> SNAMDLQLSKRLQKVANYVPKGARLLDVGSDHAYLPIFLLQMGYCDFAIAGEVVNGPYQSALKNVSEHGLTSKIDVRLANGLSAFEEADNIDTITICGMGGRLIADILNNDIDK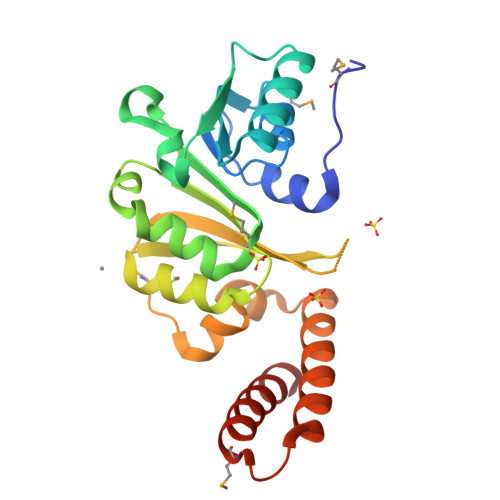LQHVKTLVLQPNNREDDLRKWLAANDFEIVAEDILTENDKRYEILVVKHGHMNLTAKELRFGPFLLSNNTTVFKEKWQNELNKLTFALNSIPNSKMEERAILEDKIQDIKEVLDES The transcriptional repressor Rex plays important roles in regulating the expression of respiratory genes by sensing the reduction–oxidation (redox) state according to the intracellular NAD+/NADH balance. Rex monitors the redox state according to the intracellular NAD+/NADH ratio and controls the Rex regulon involved in various pathways, including cellular respiration, fermentation, oxidative stress response, and biofilm formation. Structural studies of Rex family proteins have shown that Rex exists as a homodimer with N-terminal winged helix-turn-helix motifs and C-terminal NAD(H) binding motifs. The Tma Rex was composed of two distinct domains, an N-terminal DNA binding domain (residues 1–77) and a C-terminal dimerization domain (residues 84–208), which was linked by a flexible bending loop (residues 78–83).

In the present paper, we determine the crystal structure of Tma Rex dimer in complex with an operator DNA and two NAD+ molecules. The crystal structure of the ternary complex form was determined at 2.40 Å resolution and refined with crystallographic Rwork and Rfree values of 19.53% and 25.09%, respectively. The asymmetric unit contained a dimeric Rex protein bound to one molecule of NAD+ per monomer and a 22-bp DNA of TM0201 operator region (5’-ATTTGAGAAATTTATCACAAAA-3’). The N-terminal domain of Rex, including the helix-turn-helix motif, formed extensive contacts with the DNA in addition to DNA sequence specificity through electrostatic interactions and hydrogen bonds. The DNA recognition helix, α3 (residues 43–54), mainly contributed to the interaction with the major groove of DNA by hydrogen bonds. The α1 helix, α2 helix, and a strictly conserved glycine-rich winged region (residues 55–65) also supported various interactions with the DNA molecule. Residues Arg48 and Lys49 of Tma Rex were key residues for recognition of the major groove of the DNA. The NE and NH2 atoms of Arg48 played a role as hydrogen bond donors and interacted tightly with the N7 and O6 atom of Gua5, respectively. The ADP moiety of NAD+ was buried in a hydrophobic pocket (residues Val88, Val134, Leu137, Val153, Pro154, and Ile161) and bound by hydrogen bonds with residues Asn92, Ile93, Asp115, and Lys120. As a result, the distance between the central residue, Arg48, of DNA recognition helices in the ternary complex structure was 36.3 Å, which was smaller than 38.5 Å in the NAD+-bound form.

>MAEKIPKPVSKRLVSYYMCLERLLDEGVEVVSSEELARRLDLKASQIRKDLSYFGEFGKRGVGYNVEHLYDAIGEILGVKKEWKLVVVGAGNIGRAVANYTVMKEKGFRIIGIFDSDPSKIGKEAAPGLTVSDVSELEKFVEEHGVEIGVIAVPAEHAQEIAERLEKAGIKGILNFAPVKIKVSVPVENIDITASLRVLTFEIVRRNS[2x]>DGQG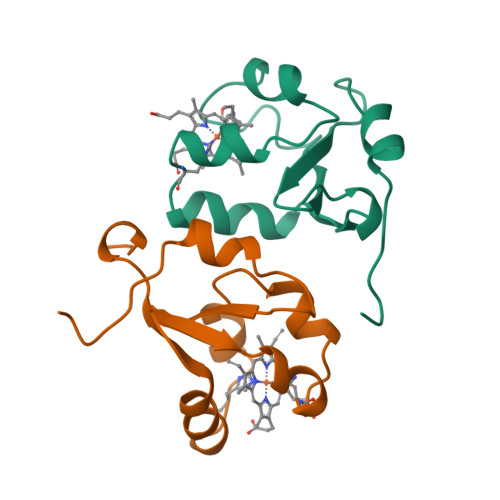SDPAVTYYRLEEVAKRNTAEETWMVIHGRVYDITRFLSEHPGGEELLLEQAGADATESFEDLGHSPDAREMLKQYYIGDVHPNDLKPK[2x]>[4x]MDDMQVYIANLGKYNEGELVGAWFTFPIDFEEVKEKIGLNDEYEEYAIHDYELPFTVDEYTSIGELNRLWEMVSELPEELQSEL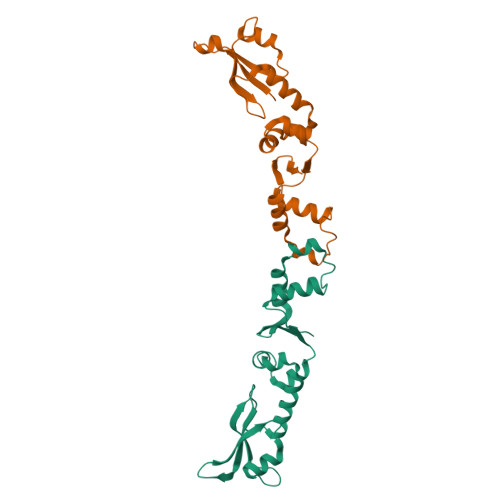SALLTHFSSIEELSEHQEDIIIHSDCDDMYDVARYYIEETGALGEVPASLQNYIDYQAYGRDLDLSGTFISTNHGIFEIVY> MSLSNTPIELKGSSFTLSVVHLHEAEPEVIRQALEDKIAQAPAFLKHAPVVINVSGLESPVNWPELHKIVTST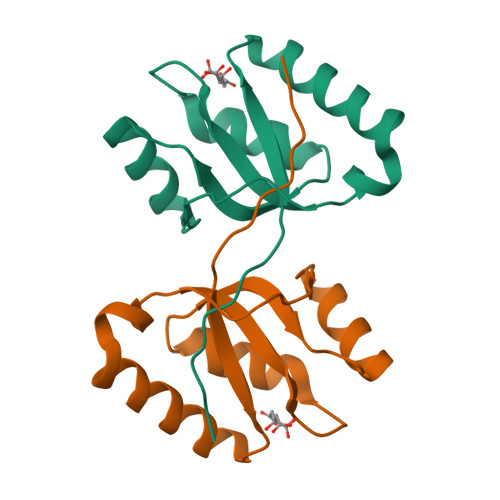GLRIIGVSGCKDASLKVEIDRMGLPLLTEGKEKAVRPAPEGHHHHHH>SEDAGLVAEAEAVAAGWMLDFLCLSLCRAFRDGRSEDFRRTRNSAEAIIHGLSSLTACQLRTIYICQFLTRIAAGKTLDAQFENDERITPLESALMIWGSIEKEHDKLHEEIQNLIKIQAIAVCMENGNFKEA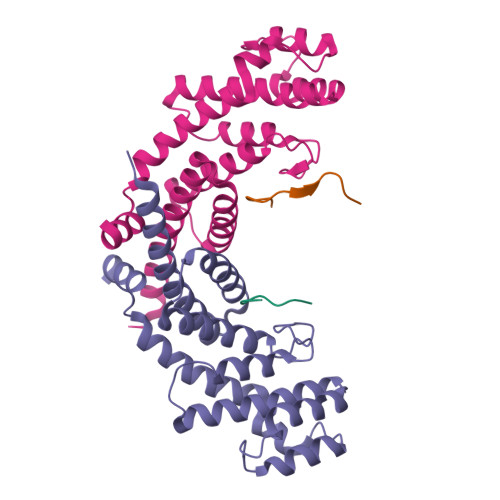EEVFERIFGDPNSHMPFKSKLLMIISQKDTFHSFFQHFSYNHMMEKIKSYVNYVLSEKSSTFLMKAAAKVVE[2x];>SKKILLTPRRRQRLS[2x]>[5x]GMDKSAKAPAITIFDHRGCSRAPKESSAKSGSQDDEMLVKVASTKVTVSEDVAAKKLQEFIGFKEKGLDGSVIRKK;>MLDAFSRVVTNADSKAAYVGGADLQA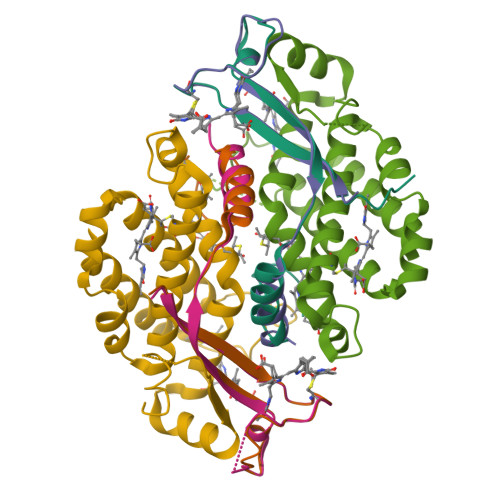LKKFISEGNKRLDAVNSIVSNASCIVSDAVSGMICENPSLISPSGNCYTNRRMAACLRDAEIILRYVSYALLSGDSSVLEDRCLNGLKETYSSLGVPANGNARAVSIMKACSVAFVNNTASQKKLSTPQGDCSGLASEVAGYFDKVTSAIS[8x];>[5x]AMDKSAKAPVITIFDHRGCSRAPKEYTGSKASGQDDEMMVKAQSVKIAVSDGVAESVLKDSLSVMHK> GEFRQNPCGSKACRRLFGPVDSEQLSRDCDALMAGCIQEARERWNFDFVTETPLEGDFAWERVR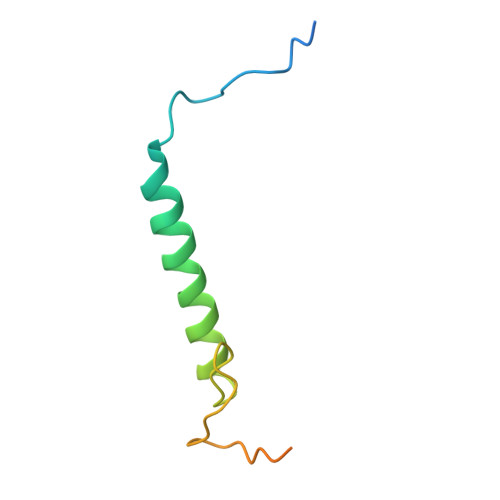GLGLPKLYLPTGPRRG>[2x]MGD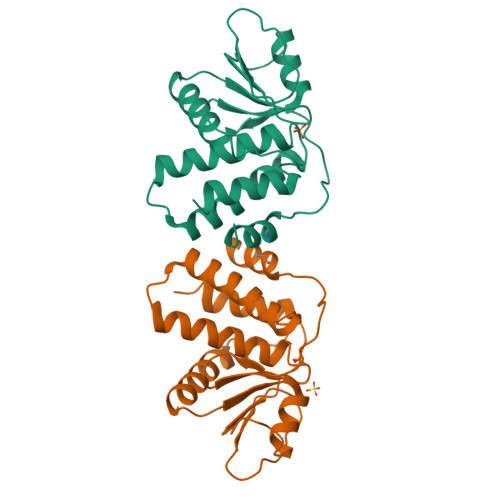KSEWYARLLLRCTRAGPPLALPSGMTRLTDHVYLGSAEDARAVLRGDSGVDFKCLVNMTMSKYSTPAGITAYHIPLRDDDKTNIASIMPALVKLLARLEAEQKPTLVHSVAGVNRSGAAAMGYVMHKRLAENPTMTQPARFVYFLKTYYEIRDLRGAFLENANFRYQLIKMFVCDSPS> MASQSSVAVISSAAARGESFPDSKKPIGSVRFQQPLRLSFSYCKSGNMSSRICAMAKPNDAETLSSSVDMSLSPRVQSLKPSKVMVITDLAATLVQSGVPVIRLAAGEPDFDTPKVVAEAGINAIREGFTRYTLNAGITELREAICRKLKEENGLSYAPDQILVSNGAVQSLLQAVLAVCSPGDEVIIPAPYWVSYTEQARLADATPVVIPTKISNNFLLDPKDLESKLTEKSRLLILCSPSNPTGSVYPKSLLEEIARIIAKHPRLLVLSDEIYEHIIYAPATHTSFASLPDMYERTLTVNGFSKAFAMTGWRLGYLAGPKHIVAACSKLQGQVSSGASSIAQKAGVAALGLGKAGGETVAEMVKAYRERRDFLVKSLGDIKGVKISEPQGAFYLFIDFSAYYGSEAEGFGLINDSSSLALYFLDKFQVAMVPGDAFGDDSCIRISYA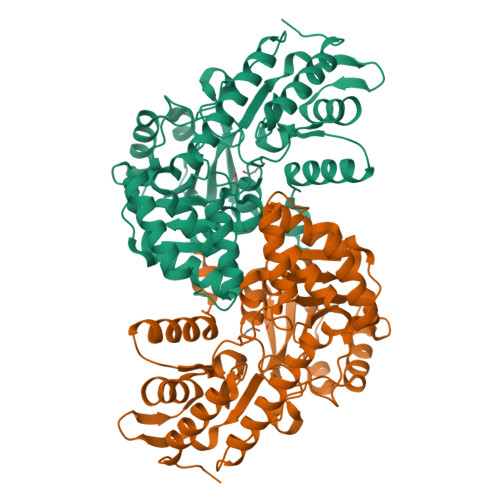TSLDVLQAAVEKIRKALEPLRATVSV>[2x]QTVPEGYQLQQVLMMSRANLRAPLANNGSVLEQSTPNKWPEWDVPGGQLTTK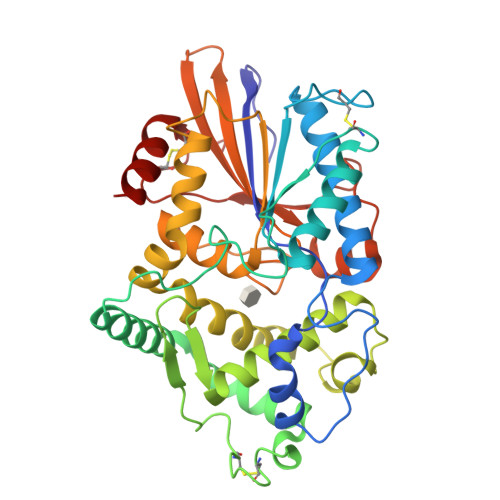GGVLEVYMGHYMREWLAEQGMVKSGECPPPYTVYAYANSLQRTVATAQFFITGAFPGCDIPVHHQEKMGTMDPTFNPVITDDSAAFSEQAVAAMEKELSKLQLTDSYQLLEKIVNYKDSPACKEKQQCSLVDGKNTFSAKYQQEPGVSGPLKVGNSLVDAFTLQYYEGFPMDQVAWGEIKSDQQWKVLSKLKNGYQDSLFTSPEVARNVAKPLVSYIDKALVTDRTSAPKITVLVGHDSNIASLLTALDFKPYQLHDQNERTPIGGKIVFQRWHDSKANRDLMKIEYVYQSAEQLRNADALTLQAPAQRVTLELSGCPIDADGFCPMDKFDSVLNEAVK(2S)-N-[(1R,2S,3S,4R,5S)-4-[(2R,3R,4S,5S,6R)-6-(aminomethyl)-3,4,5-tris(oxidanyl)oxan-2-yl]oxy-5-azanyl-2-[(2S,3R,4S,5S,6R)-4-azanyl-6-(hydroxymethyl)-3,5-bis(oxidanyl)oxan-2-yl]oxy-3-oxidanyl-cyclohexyl]-4-azanyl-2-oxidanyl-butanamide | C22 H43 N5 O13 | 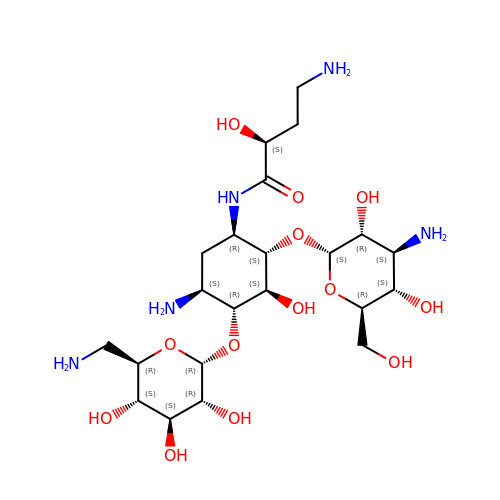LKCWBDHBTVXHDL-RMDFUYIESA-N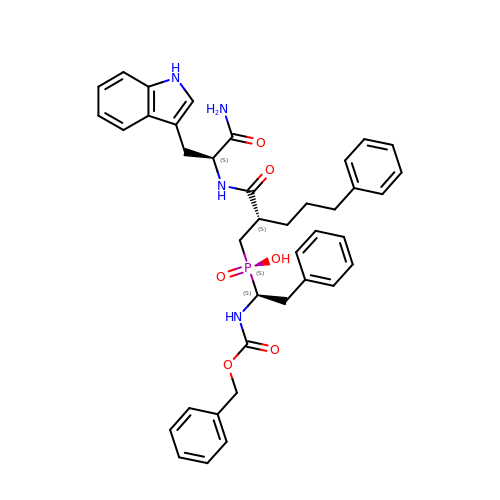1-BENZYLOXYCARBONYLAMINO-2-PHENYL-ETHYL)-{2-[1-CARBAMOYL-2-(1H-INDOL-3-YL)-ETHYLCARBAMOYL]-5-PHENYL-PENTYL}-PHOSPHINIC ACID | C39 H43 N4 O6 P | YQEMFOGNUTYMTJ-JNBVYXHXSA-N> MASTKSELIERLATQQSHIPAKTVEDAVKEMLEHMASTLAQGGSGGLTKAEMSEYLFDKLGLSKRDAKELVELFFEEIRRALENGEQVKLSGFGNFDLRDKNQRPGRNPKTGEDIPITARRVVTFRPGQKLKSRVENAGGGERIEI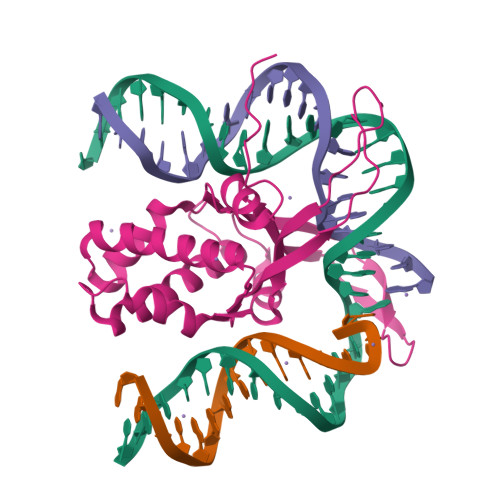RGFGSFSLHYRAPRTGRNPKTGDKVELEGKYVPHFKPGKELRDRANIYGGSGHHHHHH>[3x]SMTDLLSAEDIKKAIGAFTAADSFDHKKFFQMVG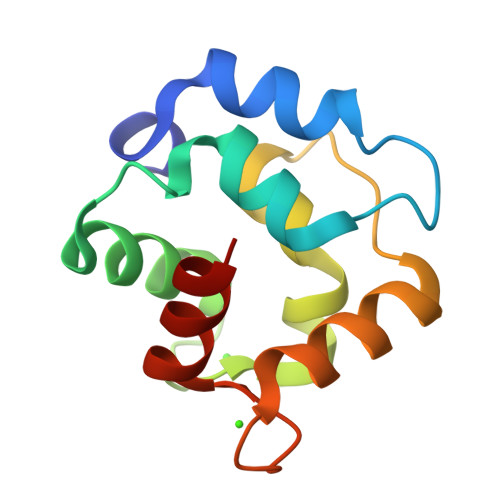LKKKSADDVKKVFHILDKDKSGFIEEDELGSILKGFSSDARDLSAKETKTLMAAGDKDGDGKIGVEEFSTLVAES>MKVMIEKILLVQTLKRLPRMGWLIKGVQEPESIADHSFGVAFITLVLADVLEKRGKRIDVEKALKMAIVHDLAEAIITDIPLSAQEFVDKDKAEALVFKKVFPEFYELYREYQECSSPEAQLVRIADKLDMILQAYQYELSG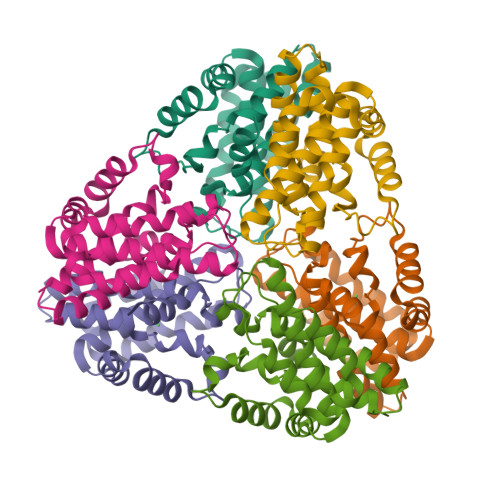NKNLDEFWEAIEEIKRLELSKYLEDILNSVGRLKA[6x]>[2x]AEAGITGTWYNQLGSTFIVTAGADGALTGTYE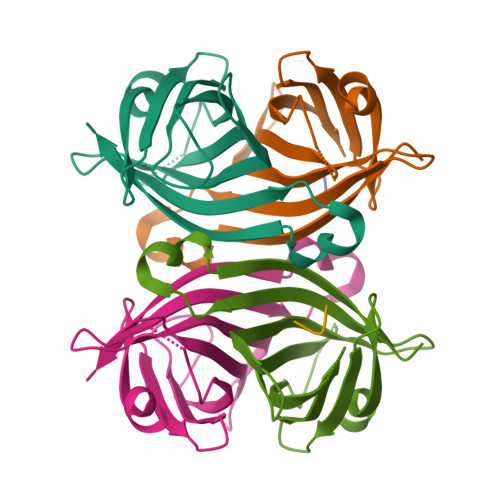SAVGNAESRYVLTGRYDSAPATDGSGTALGWTVAWKNNYRNAHSATTWSGQYVGGAEARINTQWLLTSGTTEANAWKSTLVGHDTFTKV;> FSHPQNT>MADKELKFLVVDDFSTMRRIVRNLLKELGFNNVEEAEDGVDALNKLQAGGYGFVISDWNMPNMDGLELLKTIRADGAMSALPVLMVTAEAKKENIIAAAQAG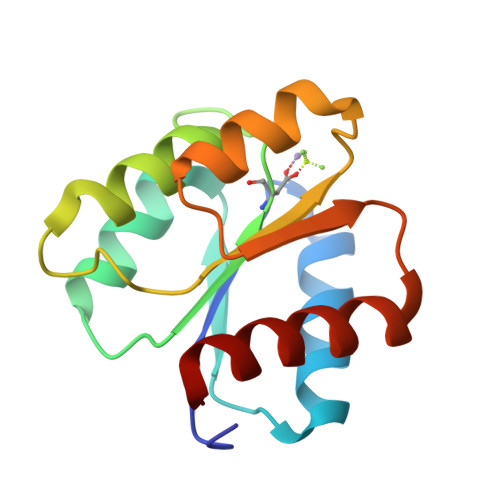ASGYVVKPFTAATLEEKLNKIFEKLGM[2x]Nucleases of the S1/P1 family have important applications in biotechnology and molecular biology. We have performed structural analyses of SmNuc1 nuclease from Stenotrophomonas maltophilia, including RNA cleavage product binding and mutagenesis in a newly discovered flexible Arg74‐motif, involved in substrate binding and product release and likely contributing to the high catalytic rate. The activity of SmNuc1 towards c‐di‐GMP in crystal resulted in a distinguished complex with the emerging product 5′‐GMP. This enzyme from an opportunistic pathogen relies on specific architecture enabling high performance under broad conditions, attractive for biotechnologies.

Purine nucleotide binding differs compared to pyrimidines, confirming the plasticity of the active site. The enzyme–product interactions indicate a gradual, stepwise product release.

>[2x]WGAQGHRLVAEVADARLNPTARAEVDRLLATEPDATLASIAPWADQLRAKDPGLGRRSAGWHYVNIAEDNCHYEAPKHCRNGNCIVEALKAQSTILGDRSLTDGERLQALKFVVHLVGDIHQPMHAGYAHDKGGNDFQLQFGNRGTNLHSLWDSGMLNTRKLDDAGYLPLLQSQRAPKLARQSNPQRDPQTWAEASCRISMQAGVYPATRKIGDEYTERYRPLAEAQLRLAGENLAQLLNRVLGARLEHHHHHH>GAQAEVRIDGPIEYGVFESRYQDFQPGERVLTRSEQNIQQ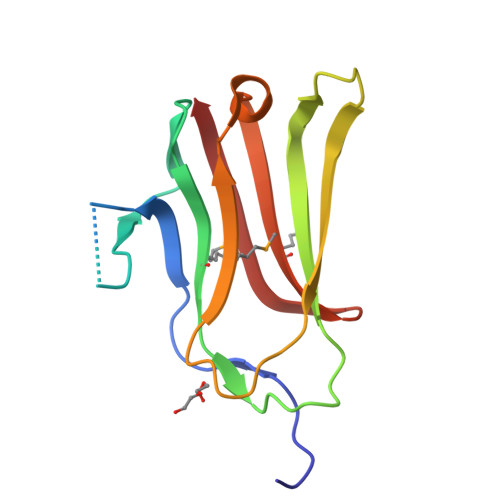TTEVPAKLGTKFGMRYQLSGKQEGDTPLTLLYLTPGVVTPDGQRHDKFEVVQKLVPGAPTDVMAYEFTEPHEVVKGEWRLMVFQGDRLLAEKSFDVR[2x]>SSYRQARWWAQEITELAQGPGRDFLQLHRHDSYAPPRPGTLARWFVNGAGYFAAVADAILRAQEEIFITDWWLSPEVYLKRPAHSDDWRLDIMLKRKAEEGVRVSILLFKEVELALGINSGYSKRALMLLHPNIKVMRHPDQVTLWAHHEKLLVVDQVVAFLGGLDLAYGRWDDLHYRLTDLGDSSESAASQPPTPRPDSPATPDLSHNQFFWLGKDYSNLITKDWVQLDRPFEDFIDRETTPRMPWRDVGVVVHGLPARDLARHFIQRWNFTKTTK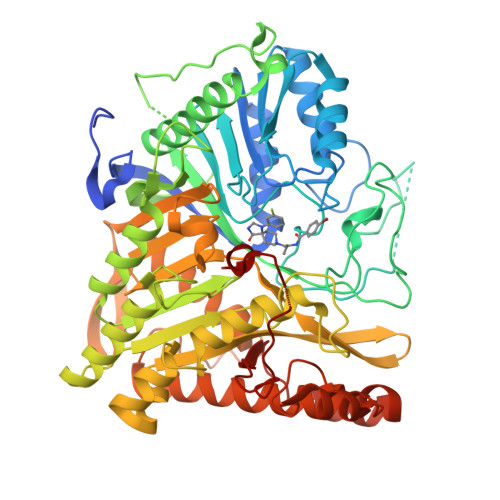AKYKTPTYPYLLPKSTSTANQLPFTLPGGQCTTVQVLRSVDRWSAGTLENSILNAYLHTIRESQHFLYIENQFFISCSDGRTVLNKVGDEIVDRILKAHKQGWCYRVYVLLPLLPGFEGDISTGGGNSIQAILHFTYRTLCRGEYSILHRLKAAMGTAWRDYISICGLRTHGELGGHPVSELIYIHSKVLIADDRTVIIGSANINDRSLLGKRDSELAVLIEDTETEPSLMNGAEYQAGRFALSLRKHCFGVILGANTRPDLDLRDPICDDFFQLWQDMAESNANIYEQIFRCLPSNATRSLRTLREYVAVEPLATVSPPLARSELTQVQGHLVHFPLKFLEDESLLPPLGSKEGMIPLEVWT[4x]> MGSSHHHHHHSSGETVRFQGHMRNPAMYSEEARLKSFQNWPDYAHLTPRELASAGLYYTGIGDQVQCFACGGKLKNWEPGDRAWSEH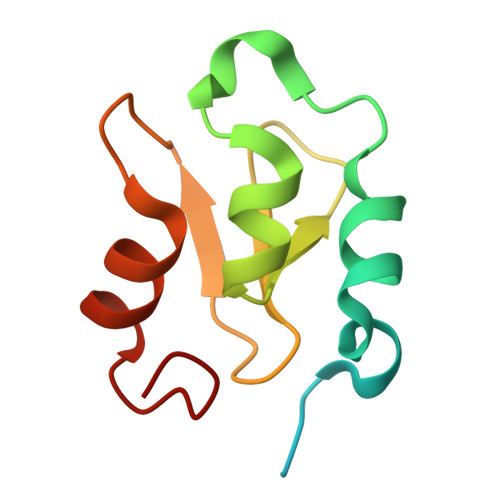RRHFPNCFFVL>SNAMKVAVIMGSSSDWKIMQESCNMLDYFEIP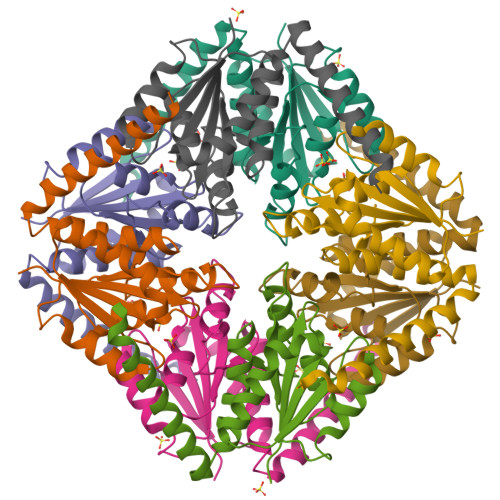YEKQVVSAHRTPKMMVQFASEARERGINIIIAGAGGAAHLPGMVASLTTLPVIGVPIETKSLKGIDSLLSIVQMPGGIPVATTAIGAAGAKNAGILAARMLSIQNPSLVEKLNQYESSLIQKVEDMQNELQ[8x]>MDYKDHDGDYKDHDIDYKDDDDKLALSMSSGPATTEGFGSACFKGAVADKYLSKYGESSTLLANGKWTKDMAKADIVAKAVLDWAVENGASVYCHWFQPMGSSGVRHGNSGQVHQSMFNFAEDGTPYYSFTGEQLLQGETDGSSFPNGGMRATHTAGGYLSIDPYSPIFLREDTVFIPAAFVSYNGDALDEKTPLHRATDALDKQTKRMLKAMKYDVGSASVYANIGLEQEIFLTPRHAFYRRPDLQFTGRTITGKFPARGQEMSDHYMAPISRATGAFECMRQIQQECFKMGIPLKTRHREVAPNQYEFAPMFGNAISQVDQNLMIMQVIEEVASEHGLAALLQEKPFAGVNGSGKHNNWSIGTSDGLNLMNPKQVNAKTGNPEIFPLVMAAMVSAVDKHGDLMRAAIASPGNDFRLGAMEAPPAVMSTYLGPSLTEFLNTVKNGSLGEYAPKKKPLEFGSDTLPSIEVPAEDRNRTSPFPYGGNRFEFRAAGSSQNVSLVNTVLNTIAAEAFKIVADRLEAGEKPLAIAQDLLKTHDKCIFNGNGYDPAWPDEAVKRGIWRIDAGCDAINELDSAKNVTLFEGMGIFTAREIQARKSVLLGHYVGSVEMEALTMIDMINQHVIPSVKKADLGNPSKLVDAVKTIKGAVAQI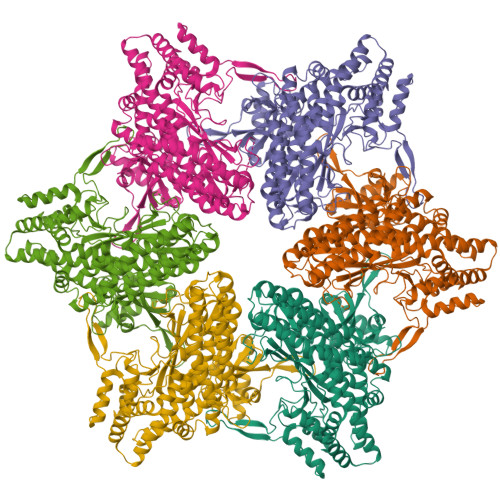HGTEDEHKAATLARTLRLTTMVAIREIIDEFESRCPPEDWTLATYSELLFFDTYPESEYGCGGGGSHHHHHHHHHH[6x]>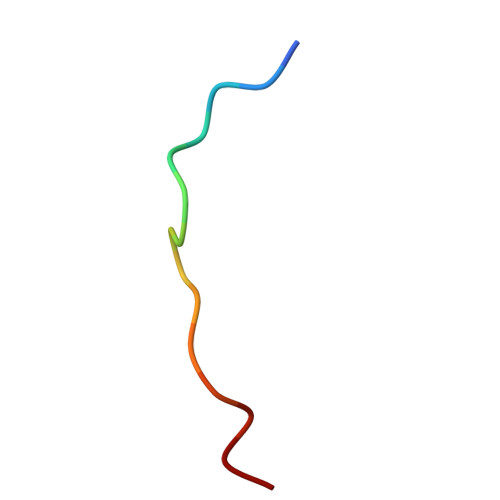 SVWIPVNEGASTSGM>GPNVCAVQKVIGTNRKYFTNCKQWYQRKICGKSTVISYECCPGYEKVPGEKGCPAALPLSNLYETLGVVGSTTTQLYTDRTEKLRPEMEGPGSFTIFAPSNEAWASLPAEVLDSLVSNVNIELLNALRYHMVGRRVLTDELKHGMTLTSMYQNSNIQIHHYPNGIVTVNCARLLKADHHATNGVVHLIDKVISTITNNIQQIIEIEDTFETLRAAVAASGLNTMLEGNGQYTLLAPTNEAFEKIPSETLNRILGDPEALRDLLNNHILKSAMCAEAIVAGLSVETLEGTTLEVGCSGDMLTINGKAIISNKDILATNGVIHYIDELLIPDSAKTLFELAAESDVSTAIDLFRQAGLGNHLSGSERLTLLAPLNSVFKDGTPPIDAHTRNLLRNHIIKDQLASKYLYHGQTLETLGGKKLRVFVYRNSLCIENSCIAAHDKRGRYGTLFTMDRVLTPPMGTVMDVLKGDNRFSMLVAAIQSAGLTETLNREGVYTVFAPTNETFRALPPRERSRLLGDAKELANILKYHIGDEI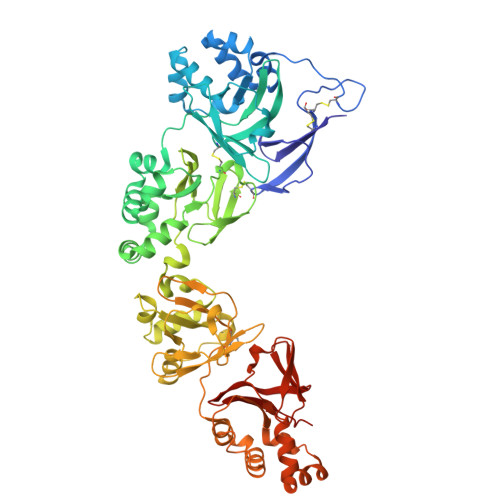LVSGGIGALVRLKSLQGDKLEVSLKNNVVSVNKEPVAEPDIMATNGVVHVITNVLQHHHHH[2x]> MKTPTFGKREETLT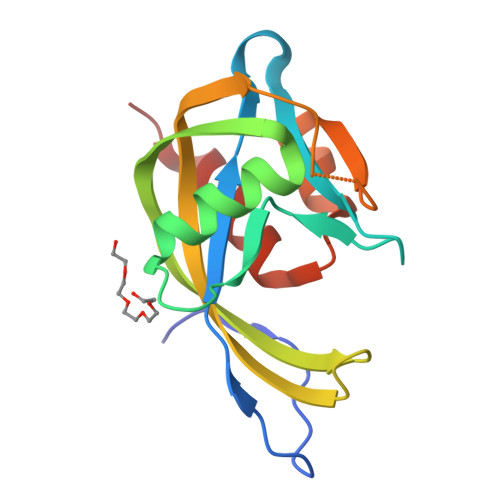YQTRYAAYIIVSKPENNTMVLVQAPNGAYFLPGGEIEGTETKEEAIHREVLEELGISVEIGCYLGEADEYFYSNHRQTAYYNPGYFYVANTWRQLSEPLERTNTLHWVAPEEAVRLLKRGSHRWAVEKWLAAAS> MKINRQQYAESYGPTVGDEVRLADTDLWIEVEKDYTTYGDEVNFGGGKVLREGMGENGTYTRTENVLDLLLTNALILDYTGIYKADIGVKDGYIVGIGKGGNPDIMDGVTPNMIVGTATEVIAAEGKIVTAGGIDTHVHFINPDQVDVALANGITTLFGGGTGPAEGS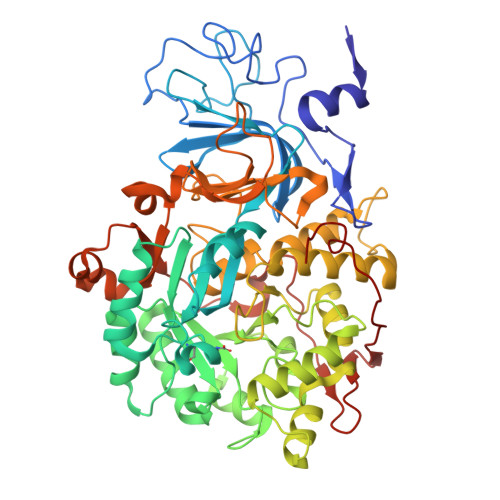KATTVTPGPWNIEKMLKSTEGLPINVGILGKGHGSSIAPIMEQIDAGAAGLKIHEDWGATPASIDRSLTVADEADVQVAIHSDTLNEAGFLEDTLRAINGRVIHSFHVEGAGGGHAPDIMAMAGHPNVLPSSTNPTRPFTVNTIDEHLDMLMVCHHLKNNIPEDVAFADSRIRPETIAAEDILHDLGIISMMSTDALAMGRAGEMVLRTWQTADKMKKQRGPLAEEKNGSDNFRLKRYVSKYTINPAIAQGIAHEVGSIEEGKFADLVLWEPKFFGVKADRVIKGGIIAYAQIGDPSASIPTPQPVMGRRMYGTVGDLIHDTNITFMSKSSIQQGVPAKLGLKRRIGTVKNCRNIGKKDMKWNDVTTDIDINPETYEVKVDGEVLTCEPVKELPMAQRYFLF>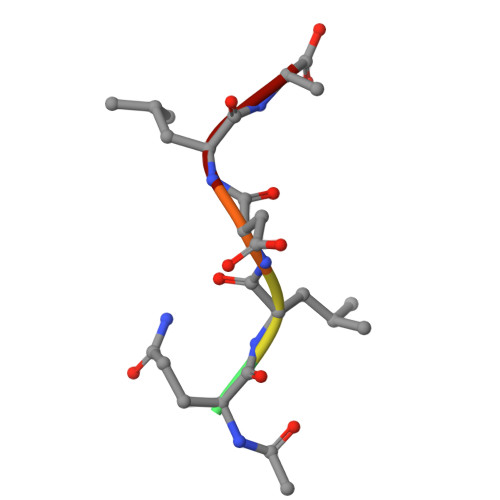 XQLDLA> MPFVNKQFNYKDPVNGVDIAYIKIPNAGQMQPVKAFKIHNKIWVIPERDTFTNPEEGDLNPPPEAKQVPVSYYDSTYLSTDNEKDNYLKGVTKLFERIYSTDLGRMLLTSIVRGIPFWGGSTIDTELKVIDTNCINVIQPDGSYRSEELNLVIIGPSADIIQFECKSFGHEVLNLTRNGYGSTQYIRFSPDFTFGFEESLEVDTNPLLGAGKFATDPAVTLAHELIHAGHRLYGIAINPNRVFKVNTNAYYEMSGLEVSFEELRTFGGHDAKFIDSLQENEFRLYYYNKFKDIASTLNKAKSIVGTTASLQYMKNVFKEKYLLSEDTSGKFSVDKLKFDKLYKMLTEIYTEDNFVKFFKVL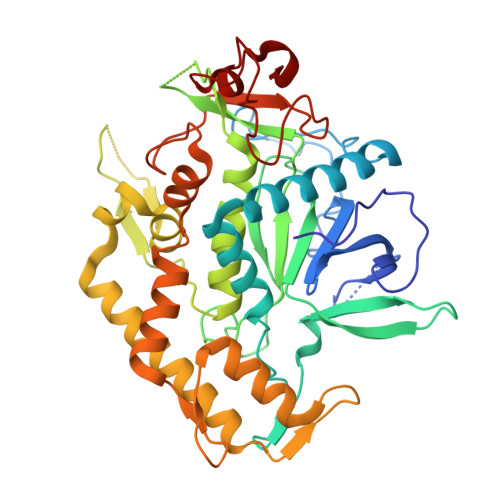NRKTYLNFDKAVFKINIVPKVNYTIYDGFNLRNTNLAANFNGQNTEINNMNFTKLK>MFNNRIRTAALAGAIAISTAASGVAIPAFAQETGTYNNTGGFNDADGSTIQPAPAVDHSEAELRDATDATGNYLAAFQSGDIEAIVGAYIDAGVDGFDPSEEAIFKAFEAARDEATQQLAFSAETITKTRESVAYALKVDQEATEAYLAYRNALRGAATSINPLIDAANAANRTDGSEIEIYDNIFLASDVFTDGPLLLPAYRELVALQTEVNEDLEWLGEFAIDNDADNYVQRYHIPAVEALKAEIDARLEAIEPLRADSAEKNRLAQKSDVLVRQLFLERATAQRDTLRIVEAIFATATRYVELYESDEDVNVEGKTLREHYFALFPTLFGAASFNVGVLNTADDAVIDYYLVWDTDLETNDEDAAYAEEKREFALLTYAKIFINGQWQEKVKYVQNLDDGARAEAARIEAERLADEAYRAEQLRIAQEAADAQKAIADALAKEAENNNNSGGDNSSDDKGTGSSDIGSWGPFAAIAAIIAAIAAIFPFLSGIVKF[6x]

Corynebacteria belong to the bacterial family Mycobacteriaceae, which is characterized by a highly unusual cell envelope with an outer membrane consisting of mycolic acids, called mycomembrane. The C. glutamicum MM is further coated with an S-layer made of the PS2 protein, which adds another level of complexity to this unusual cell envelope that is incompletely understood at the ultrastructural and molecular levels. Our structure shows that the S-layer of C. glutamicum is composed of a hexagonal array of the PS2 protein, which interacts directly with the mycomembrane via an anchoring segment containing a coiled-coil motif. PS2 is an SLP composed entirely of α-helices, an unusual feature among prokaryotic S-layers.

The resulting data was used to obtain a cryo-EM reconstruction at 3.1 Å global resolution, which allowed us to build an atomic model of the C. glutamicum PS2 S-layer. Amino acid residues 33–445 could be reliably modeled into the cryo-EM map, which was sufficient to visualize the S-layer lattice contacts. The missing N-terminal residues of PS2 (residues 1–32) are predicted to form a signal peptide for Sec-dependent secretion and are presumably cleaved off and not present in the mature SLP that forms the S-layer lattice. At the other end of the PS2 protein sequence, the missing C-terminal residues (446–498) were previously shown to be important for cell envelope anchoring and are also predicted by bioinformatic analyses to form an anchoring segment on cells. Due to detergent (SDS) treatment during S-layer purification, this anchoring segment was likely detached from the MM and remained too flexible to be resolved in our cryo-EM analysis. The PS2 monomers assemble into tight hexamers within the lattice, which in turn are linked to each other through prominent trimeric interfaces that are repeated throughout the lattice. The hexameric linkages are primarily established by residues 90–110 and 300–445, located around the center of the hexamer and in the coiled-coil MM-anchoring segment. Each hexameric unit is connected to neighboring hexamers through trimeric interfaces, mainly involving residues 194–204 and 213–235. Both the trimeric and hexameric interfaces are formed by a combination of hydrophilic and hydrophobic interactions, including salt bridges and π-stacking of aromatic side chains. The combination of hexameric and trimeric interfaces results in varying pores sizes of 6, 27, and 81 Å within the lattice.> MIIDSKTTLPRHSLIHTIKLNSNKKYGPGDMTNGNQFIISKQEWATIGAYIQTGLGLPVNEQQLRTHVNLSQDISIPSDFSQLYDVYCSDKTSAEWWNKNLYPLIIKSANDIASYGFKVAGDPSIKKDGYFKKLQDELDNIVDNNSDDDAIAKAIKDFKARCGILIKEAKQYEEAAKNIVTSLDQFLHGDQKKLEGVINIQKRLKEVQTALNQAHGESSPAHKELLEKVKNLKTTLERTIKAEQDLEKKVEYSFLLGPLLGFVVYEILENTAVQHIKNQIDEIKKQLDSAQHDLDRDVKIIGMLNSINTDIDNLYSQGQEAIKVFQKLQGIWATIGAQIENLRTTSLQEVQDSDDADEIQIELEDASDAWLVVAQEARDFTLNAYSTNSRQNLPINVISDSCNCSTTNMTSNQYSNPTTN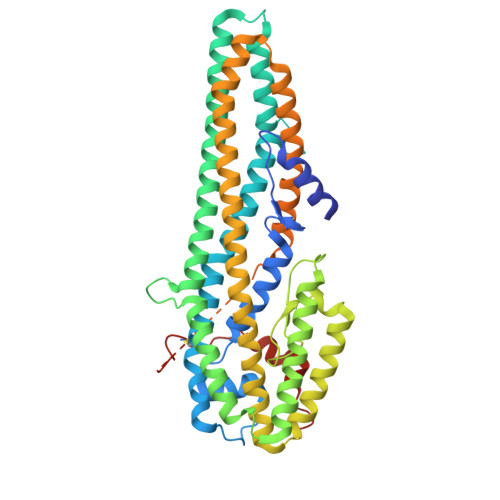MTSNQYMISHEYTSLPNNFMLSRNSNLEYKCPENNFMIYWYNNSDWYNNSDWYNN Cereblon (CRBN) is the substrate receptor of the CRL4CRBN E3 ubiquitin ligase and is a central player in targeted protein degradation. It is the target of the thalidomide-derived immunomodulatory drugs (IMiDs) and is one of the most widely employed receptors for proteolysis-targeting chimeras (PROTACs), both of which induce the ubiquitination and subsequent proteasomal degradation of target proteins. In our laboratory, we established the single-domain bacterial homologue cereblon isoform 4 from Magnetospirillum gryphiswaldense (MsCI4) for structural ligand-binding studies, which shares 35% sequence identity and <1 Å r.m.s.d. over 100 Cα atoms with the thalidomide-binding domain (TBD) of human CRBN. We grow MsCI4 crystals in complex with thalidomide, and then exchange thalidomide for the ligand in question in subsequent soaking experiments.

The IMiD iberdomide, which is about to enter Phase III clinical trials for different forms of MM, consists of an extended tail formed by a morpho­linomethyl-benzyl group connected via an oxy group to phthalimidine, which is attached to a classical glutarimide moiety. Compared with thalidomide, avadomide showed a slightly increased affinity, while a more than tenfold gain in affinity was observed for iberdomide. Most interestingly, the orientation of the protruding moiety was different in all three chains. While the glutarimide moiety shows the canonical interactions with the tri-Trp pocket, the phenyl ring is harboured in a channel formed by Glu76, Phe77 and Pro51 of MsCI4. While the glutarimide moiety of iberdomide is bound in an identical fashion in chains B and C, the protruding moiety is found in a very different orientation, filling a surface groove behind Trp85. In chain C, the orientation of the molecule could partially be influenced by crystal contacts with Ile70, Gly71 and Ala72 of the symmetry chain B. However, the protruding moiety in chain B adopts a very similar orientation, albeit being solvent-exposed with the nearest symmetry atoms more than 7 Å away, suggesting that this overall conformation is not the result of crystal-packing effects.

>MPLDAGGQNSTQMVLAPGASIFRCRQCGQTISRRDWLLPMGGDHEHVVFNPAGMIFRVWCFSLAQGLRLIGAPSGEFSWFKGYDWTIALCGQCGSHLGWHYEGGSQPQTFFGLIKDRLAEGPAD[3x]Transporters of the Nramp (Natural resistance-associated macrophage protein) family import divalent transition metal ions into cells of most organisms. In addition to the physiological substrates Fe2+ and Mn2+, Nramps can also transport toxic metals like Cd2+ and Hg2+ but exclude the abundant alkaline earth metals like Mg2+ and Ca2+. Recent bacterial Nramp structures reveal a LeuT fold, three stable conformations (outward-open, occluded, and inward-open), and identify the metal-binding site residues, including conserved aspartate, asparagine, and methionine residues. We present high-resolution structures of DraNramp in three conformations in both Mn2+-bound and metal-free states, providing the first molecular map of the entire Mn2+ transport cycle.

We obtained a structure of wildtype (WT) DraNramp in an occluded state bound to Mn2+ at 2.38 Å by soaking crystals with Mn2+ (WT•Mn2+). We resolved a comparable structure using co-crystallization with Mn2+ and the inward-locking mutation A47W (A47W•Mn2+; Cα RMSD=0.47 Å; all pairwise RMSD values listed in Supplementary file 1c; Bozzi et al., 2016b). The similarity of both structures, including a nearly identical Mn2+-coordination sphere, suggests that the observations we make based on these two structures are robust. Although the inner vestibule is occluded in both structures, WT•Mn2+ and A47W•Mn2+ differ in their TM1a position, with WT•Mn2+ nearly identical to G45R whereas the A47W•Mn2+ TM1a is displaced within the inner vestibule, likely to accommodate the bulky tryptophan sidechain. The conformation-locking mutants—A47W, which is outward-closed and crystallized in an occluded state, and outward-open G223W —also show different behavior with Mn2+ and Cd2+. ITC with Mn2+ agrees with the structural data, with two-site fit for A47W, and one-site fit for A47W-D296A, A47W-D369A, and G223W (assigned to the orthosteric site). However, with Cd2+, the ITC data for A47W fit best with a one-site model and we observed no binding with A47W-D296A, A47W-D369A, and G223W, indicating that there is no significant affinity for Cd2+ at the orthosteric site of A47W and G223W. (C–D) Double mutants of A47W with either D296A (C) or D369A (D) retain Mn2+ binding but not Cd2+ binding, indicating that Cd2+ binds only at the external site and not the orthosteric site of the A47W construct, whereas Mn2+ binds at both binding sites.

> MHHHHHHHHMDSRSPSLPDDRPDPPEQHLDARAGATLRGTAGPRGVRRILPFLGPWVIASIAYMDPGNFATNIEGGARYGYSLLWVILAANLMAMVIQNLSANLGIASGRNLPELIRERWPRPLVWFYWIQAELVAMATDLAEFLGAALAIQLLTGLPMFWGAVVTGVVTFWLLNLQKRGTRPLELAVGAFVLMIGVAYLVQVVLARPDLAAVGAGFVPRLQGPGSAYLAVGIIGATVMPHVIYLHSALTQGRIQTDTTEEKRRLVRLNRVDVIAAMGLAGLINMSMLAVAAATFHGKNVENAGDLTTAYQTLTPLLGPAASVLFAVALLASGLSSSAVGTMAGDVIMQGFMGFHIPLWLRRLITMLPAFIVILLGMDPSSVLILSQVILCFGVPFALVPLLLFTARRDVMGALVTRRSFTVIGWVIAVIIIALNGYLLWELLGG N-(4-{[(2-amino-4-oxo-3,4-dihydropteridin-6-yl)methyl]amino}-2-hydroxybenzene-1-carbonyl)-L-glutamic acid | C19 H19 N7 O7 | 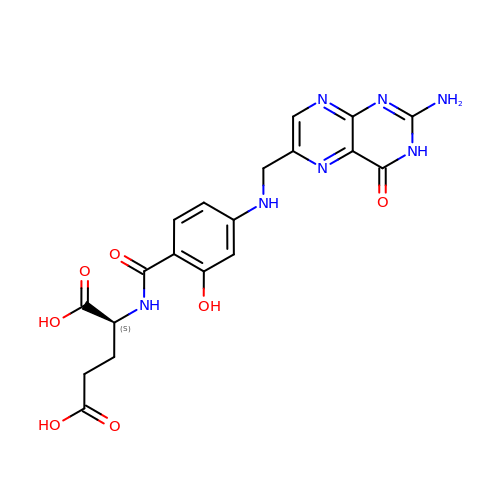WEDDXRUKABMRIT-NSHDSACASA-N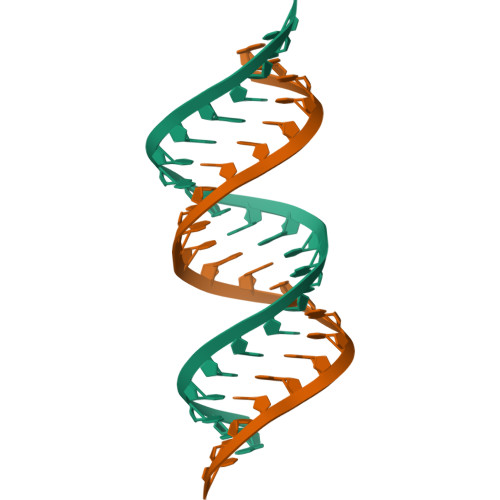> GGGCCAGCAGCAGCAGCAGGUCC> ASMTGGQQMGAPITAYAQQTRGLLGCIITSLTGRDKNQVEGEVQIVSTATQTFLA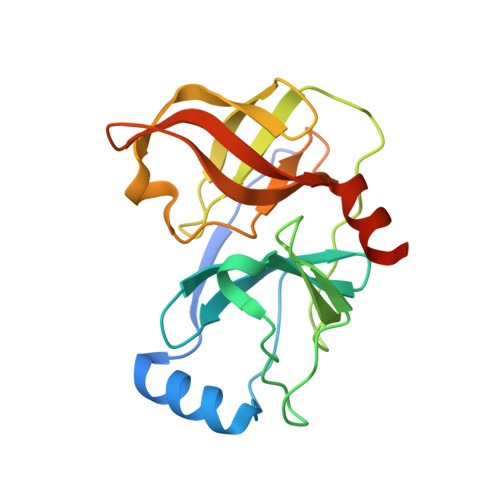TCINGVCWTVYHGAGTRTIASPKGPVIQMYTNVDQDLVGWPAPQGSRSLTPCTCGSSDLYLVTRHADVIPVRRRGDSRGSLLSPRPISYLKGSAGGPLLCPAGHAVGLFRAAVCTRGVAKAVDFIPVENLETTMRGSHHHHHH>[4x]SMSRAAFAWEDPFLLEEQLTEDERMIRDSAKAFASDVLLPRVEKAYLEETTDPELFHLMGQAGLLGVTLPEDYGAANASYVAYGLVAREVERIDSGYRSMMSVQSSLVMYPIYAYGSDEQRKKYLPGLVSGELIGCFGLTEPDAGSDPAGMKTRAEKIDGGYRLSGSKMWISNSPIADVFVVWAKSAAHDNAIRGFILEKGMKGLSAPKIGGKLSLRASITGEIV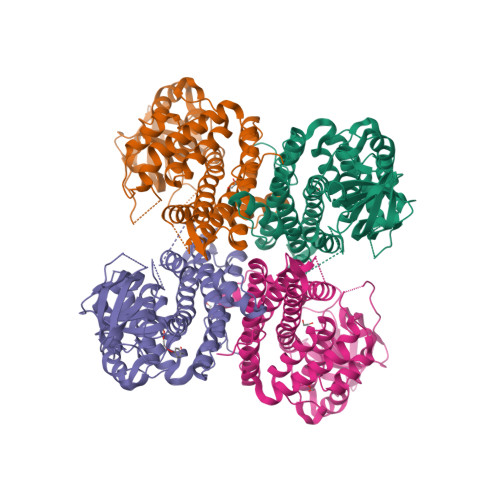MDGVEVSEDAILPNVSGLKGPFGCLNRARYGISWGVLGAAEDCWFRARQYGLDRKQFNKPLAGTQLYQKKLADMQTEIALGIQASLRVGRLFDEGKMAPEMISIVKRNNCGKALDIARQARDMHGGNGIQIEYHVMRHAQNLETVNTYEGTHDVHALILGRAQTGIQAFF>[2x]MAKKTPPVVFHWFPFIGSTISYGIDPYKFFFDCRAKYGDIFTFILLGKKTTVYLGTKGNDFILNGKLRDVCAEEVYS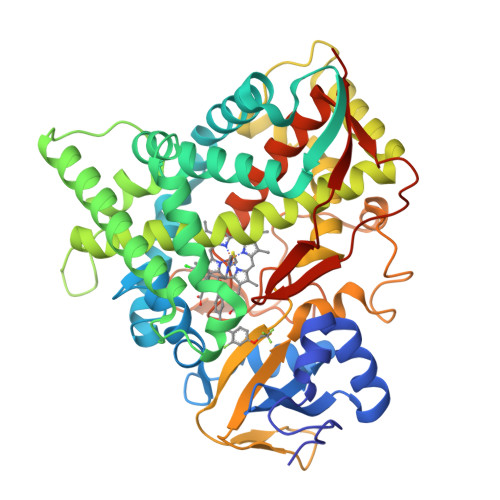PLTTPVFGRHVVYDCPNAKLMEQKKFVKYGLTSDALRSYVPLITDEVESFVKNSPAFQGHKGVFDVCKTIAEITIYTASRSLQGKEVRSKFDSTFAELYHNLDMGFAPINFMLPWAPLPHNRKRDAAQRKLTETYMEIIKARRQAGSKKDSEDMVWNLMSCVYKNGTPVPDEEIAHMMIALLMAGQHSSSSTASWIVLRLATRPDIMEELYQEQIRVLGSDLPPLTYDNLQKLDLHAKVIKETLRLHAPIHSIIRAVKNPMAVDGTSYVIPTSHNVLSSPGVTARSEEHFPNPLEWNPHRWDENIAASAEDDEKVDYGYGLVSKGTNSPYLPFGAGRHRCIGEQFAYLQLGTITAVLVRLFRFRNLPGVDGIPDTDYSSLFSKPLGRSFVEFEKRHHHHH>[4x]GANRTLIVTTILEEPYVMYRKSDKPLYGNDRFEGYCLDLLKELSNILGFLYDVKLVPDGKYGAQNDKGEWNGMVKELIDHRADLAVAPLTITYVREKVIDFSKPFMTLGISILYRKGTPIDSADDLAKQTKIEYGAVRDGSTMTFFKKSKISTYEKMWAFMSSRQQSALVKN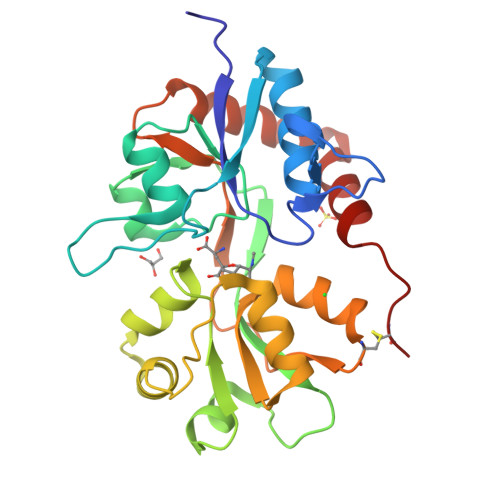SDEGIQRVLTTDYALLMESTSIEYVTQRNCNLTQIGGLIDSKGYGVGTPIGSPYRDKITIAILQLQEEGKLHMMKEKWWRGNGCP> MADYKDDDD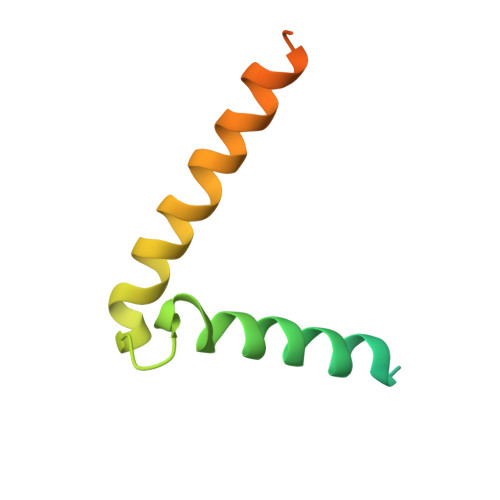KSGPDEVDASGRMAGMALARAWKQMSWFYYQYLLVTALYMLEPWERTVFNSMLVSIVGMALYTGYVFMPQHIMAILHYFEIVQ>XGE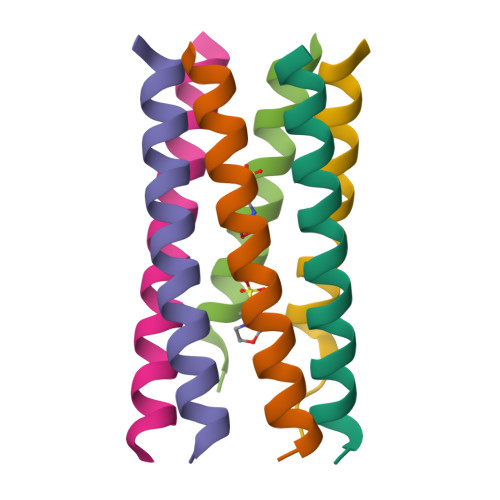LKAIAQELKAIAKELKAIAWEEKAIAQGX[6x]> QNLDSMLHGTGMKSD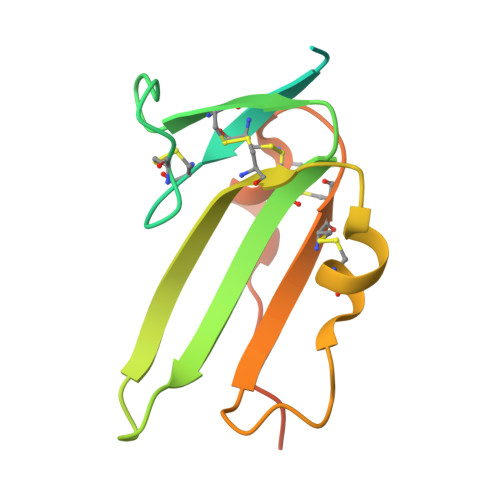SDQKKSENGVTLAPEDTLPFLKCYCSGHCPDDAINNTCITNGHCFAIIEEDDQGETTLASGCMKYEGSDFQCKDSPKAQLRRTIECCRTNLCNQYLQPTLPPVVIGPFFDGSIR>MAHHHHHHMHIHKIQAREILDSRGNPTIEADVTLTTGIIGRASVPSGASTGSREACELRDNDPKRYAGKGVQKAVKHVNNEINQALQGLSVEDQENLDRILCQLDNTENKSHLGANAILATSLACARARALSLNQPLYMTLNQGDMMTMPVPMMNILNGGAHADNNVDIQEFMIMPIGAPDFPVALQMGTEIFHVLKSVLKKQGLNTAVGDEGGFAPNIQSNRQALDLLSEAIEKAGFRLGEDIVFALDVAASELFNEGFYHMYSENQKFDSHQLIEYYANLISSYP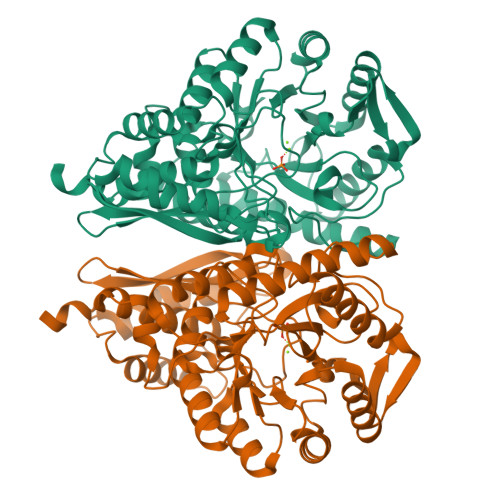IVSIEDGLDEKDWSGWKQLTTHLGNKVQLVGDDLFVTNPKILREGIAQGIANAILIKVNQIGTLSETRQAIKLAYDNGYRCVMSHRSGETEDTFIADLAVASGCGQIKTGSLCRTDRTAKYNQLLRINELASLPYAGKNILKR[2x]3-[1-[4,4-bis(4-fluorophenyl)butyl]piperidin-4-yl]-1~{H}-benzimidazol-2-one | C28 H29 F2 N3 O 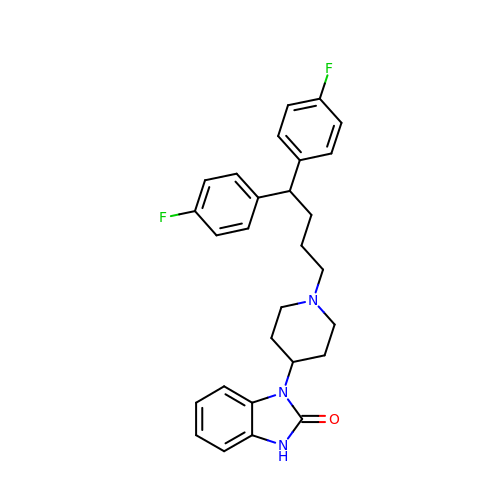| YVUQSNJEYSNKRX-UHFFFAOYSA-N> GAMGIRNSIFRKPQPFEYEGTDTGVVLLHAYTGSPNDMNFMARALQRSGYGVYVPLFSGHGTVEPLDILTKGNPDIWWAESSAAVAHMTAKYAKVFVFGLSLGGIFAMKALETLPGITAGGVFSSPIL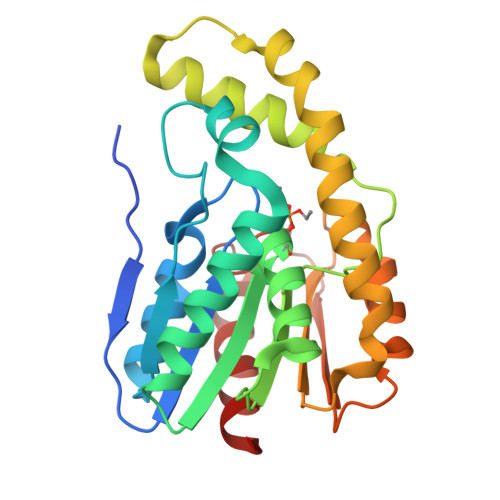PGKHHLVPGFLKYAEYMNRLAGKSDESTQILAYLPGQLAAIDQFATTVAADLNLVKQPTFIGQAGQDELVDGRLAYQLRDALINAARVDFHWYDDAKHVITVNSAHHALEEDVIAFMQQENEG>GGACUCGAAUCC[12x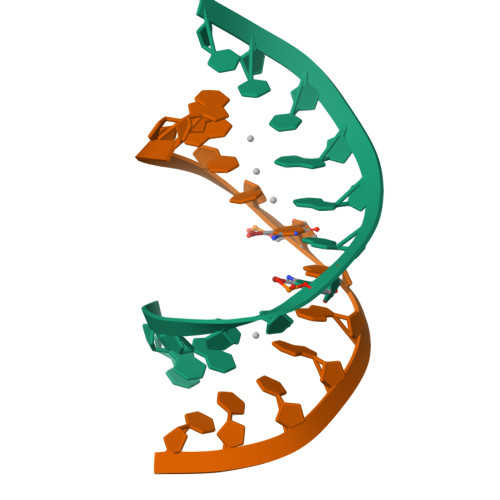]MDHAR reduces the monodehydroascorbate (MDHA) radical to AsA at the expense of an NAD(P)H molecule, with NADH being the preferred donor. We report, for the first time, the crystal structure of MDHAR of O. sativa L. japonica (OsMDHAR) to understand its detailed mechanism. Structural comparison of OsMDHAR to other proteins, using the DALI server, indicated that it has the same fold as that of putidaredoxin reductase (Pdr), biphenyl dioxygenase (BphA4)18 and rubredoxin reductase (RdxR). All these proteins consist of three domains: an NAD(P)-binding domain, an FAD-binding domain, and a C-terminal domain, as shown in Figs 1 and 2.

Except for the crystals of apo OsMDHAR and the OsMDHAR-NAD complex, which have one molecule in the asymmetric unit, there were two molecules in the asymmetric unit of the crystals. The residues participating in the van der Waals interactions with FAD are Gly13, Gly15, Ala122, Thr123, Gly297, and Ala319. Lys53, salt-bridged with Glu178, participates in hydrogen bond formation with O4 of FAD, which is also hydrogen bonded with the carbonyl oxygen of Pro49. The conserved residue Asp298 forms a hydrogen bond with O3’ of the ribitol moiety and the phosphate group is stabilized by hydrogen-bond interactions with Arg48 and Arg147. The Glu41 and Glu148 residues are hydrogen bonded with the O3B and O2B atoms of the adenosine moiety of FAD, respectively. The superposed structures show that the unique long loop of 63–80 residues of OsMDHAR is adjacent to the iron cluster of Pdx, BphA3, and Rdx, and occupies a part of the partner proteins in the complexed structures. It is involved in the formation of a closed and narrow active site pocket with positively charged residues, which only accommodates small molecules such as MDHA. In both apo and NADH complex structure, Tyr349 formed hydrogen bonds with two water molecules, whose position was corresponded to the bound substrate ligand in the AsA complex structure.

> HHHHHHASENLYFQGAMVMASEKHFKYVILGGGVAAGYAAREFAKQGVKPGELAIISKEAVAPYERPALSKGYLFPQNAARLPGFHVCVGSGGERLLPEWYSEKGIELILSTEIVKADLASKTLTSAVGATFTYEILIIATGSSVIKLSDFGTQGADSNNILYLREVDDADKLVAAIQAKKGGKAVIVGGGYIGLELSAALKINDFDVTMVFPEPWCMPRLFTADIAAFYESYYTNKGVKIVKGTVAVGFDADANGDVTAVNLKNGSVLEADIVVVGVGGRPLTTLFKGQVAEEKGGIKTDAFFETSVPGVYAVGDVATFPMKMYNELRRVEHVDHARKSAEQAVKAIKGKESGESVVEYDYLPYFYSRSFDLGWQFYGDNVGDTILFGDSDPTSAKPKFGSYWIKDGKVLGAFLEGGSPDENKAIAKVAKTQPPVANIEELKKEGLQFASKI>[4x]ATVAPDTRSLDEIYQSALKEGGTVTVYAGGDVQSQQAGFKQAFENRFPGIKLNVIVDYSKYHDARIDNQLATDTLIPDVVQLQTVQDFPRWKKQGVLLNYKPVGWDKVYPEFRDADGAWIGAYVIAFSNLVNTQLLNEKSWPREANDYLRPDLKGNLILAYPNDDDAVLFWYKQIVDKYGWEFVEKLQEQDPVYVRGTNVPGAQITTGKYSATFTSSGALVPAAG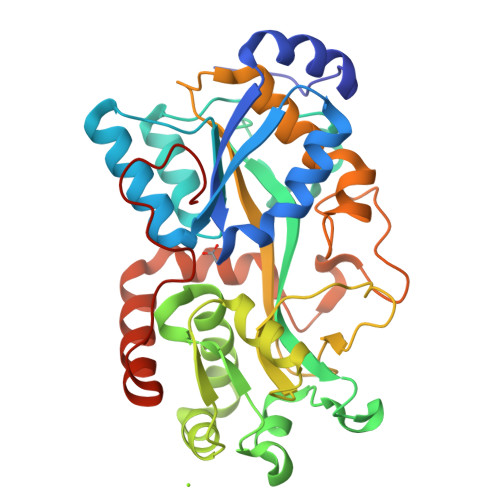SVTRFVLPKTDPFVSWAQRAAIFKQAKHPESAKLYLSWLLDPQTQTQVSRMWSVRTDVAPPAGYKHIWEYSNTRPQAFADFMSDRGAVERFRAQMSLYVGEAKGDPTPGWLGLHPEVPLA> PKAQDDSTPDSLFAGLVGEYYGTNSQLNNISDFRALVDSKEADATFEAANISYGRGSSDVAKGTHLQEFLGSDASTLSTDPGDNTDGGIYLQGYVYLEAGTYNFKVT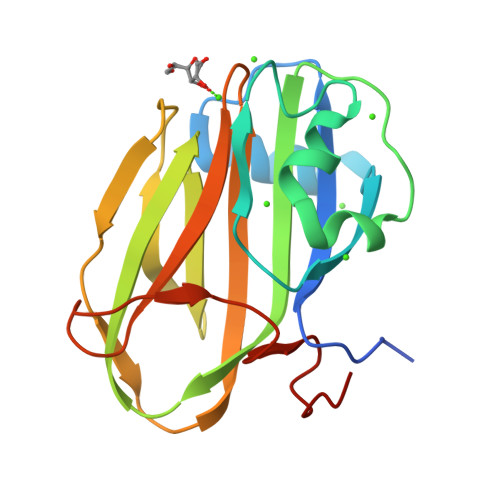ADDGYEITINGNPVATVDNNQSVYTVTHASFTISESGYQAIDMIWWDQGGDYVFQPTLSADGGSTYFVLDSAILSSTGETPYTTAQ> 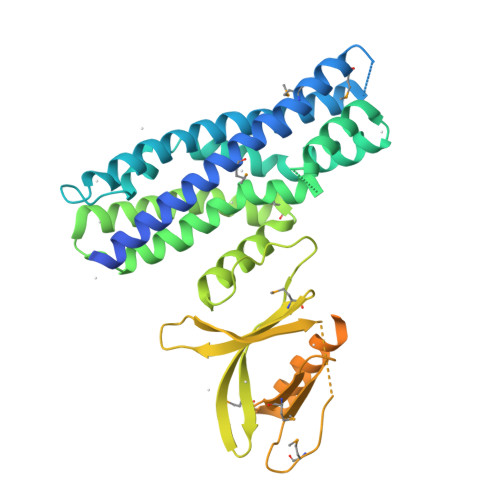MHHHHHHSSGRENLYFQGGQSRALVIAQELLSSEKAYVEMLQHLNLDFHGAVMRALDDMDHEGRDTLAREELRQGLSELPAIHDLHQGILEELEERLSNWESQQKVADVFLAREQGFDHHATHILQFDRYLGLLSENCLHSPRLAAAVREFEQSVQGGSQTAKHRLLRVVQRLFQYQVLLTDYLNNLCPDSAEYDNTQGALSLISKVTDRANDSMEQGENLQKLVHIEHSVRGQGDLLQPGREFLKEGTLMKVTGKNRRPRHLFLMNDVLLYTYPQKDGKYRLKNTLAVANMKVSRPVMEKVPYALKIETSESCLMLSASSCAERDEWYGCLSRALPEDYKAQALAAFHHSVEIRERLGVSLGERPPTLVPVTHVMMCMNCGCDFSLTLRRHHCHACGKIVCRNCSRNKYPLKYLKDRMAKVCDGCFGELKKRG>MGSSHHHHHHSSENLYFQGHMSSLPITDRKIRFGLVGCGRISKNHIGAIAQHGDRAELVEICDTNPEALQAAEAATGARPFSSLSDMLAQGNADALVLATPSGLHPWQAIEVAQAGRHVVSEKPMATRWEDGKRMVKACDEAGVRLFVVKQNRRNATLQLVKKAIEQGRFGRIYMVTVNVFWTRPQEYYDAARWRGKWEWDGGAFMNQASHYVDLLDWLVGPVESVYAYTATLARRIEAEDTGVAALRWRHGAMGSINVTMLTYPQNLEGSITILGEKGTVRVG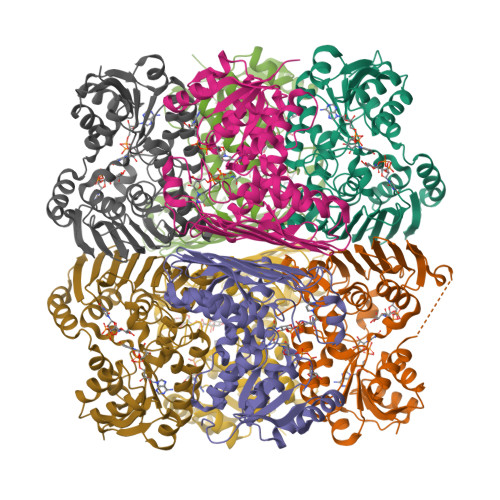GVAVNRIDEWKFAEPHPDDDKIREANYETTSVYGFGHPLYYDNVINCLRGDCEPETDGREGLQSLALLTAIYRSARDGVRIPLPLD[16x]> XTIVALKYPGGVVMAGDRRSTQGNMISGRDVRKVYITDDYTATGIAGTAAVAVEFARLYAVELEHYEKLEGVPLTFAGKINRLAIMVRGNLAAAMQGLLALPLLAGYDIHASDPQSAGRIVSFDAAGGWNIEEEGYQAVGSGSLFAKSSMKKL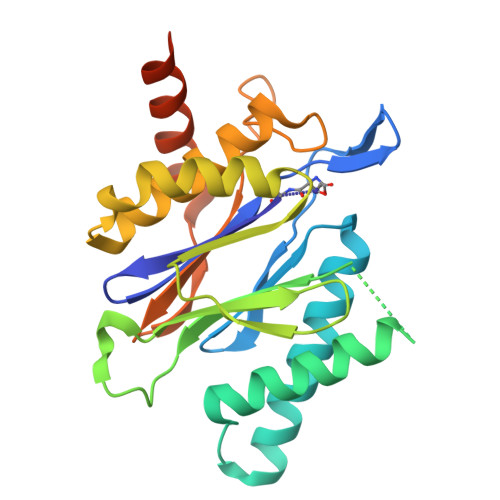YSQVTDGDSGLRVAVEALYDAADDDSATGGPDLVRGIFPTAVIIDADGAVDVPESRIAELARAIIESRSGADTFGSDGGEKHHHHHH> DADKLPHTKVTLVAPPQVHPHEQATKSGPKVVEFTMTIEEKKMVIDDKGTTLQAMTFNGSMPGPTLVVHEGDYVQLTLVNPATNAMPHNVDFHGATGALGGAKLTNVNPGEQATLRFKADRSGTFVYHCAPEGMVPWHVVSGMSGTLMVLPRDGLKDPQGKPLHYDRAYTIGEFDLYIPKGPDGKYKDYATLAESYGDTVQVMRTLTPSHIVFNGKVGALTGANALTAKVGETVLLIHSQANRDTRPHLIGGHGDWVWETGKFANPPQRDLETWFI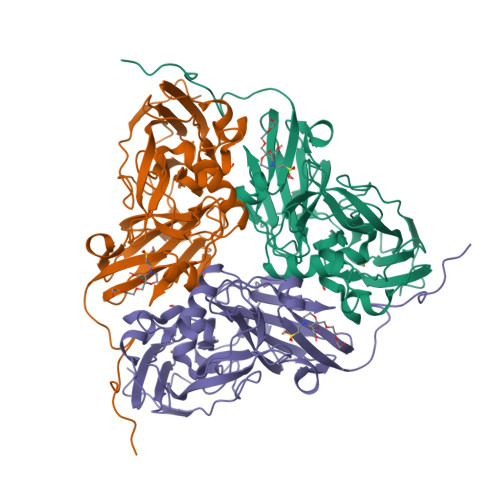RGGSAGAALYTFKQPGVYAYLNHNLIEAFELGAAGHIKVEGKWNDDLMKQIKAPAPIPR3-{5-[(2-fluorophenyl)amino]-1H-indazol-1-yl}-N-(3,4,5-trimethoxyphenyl)benzamide | C29 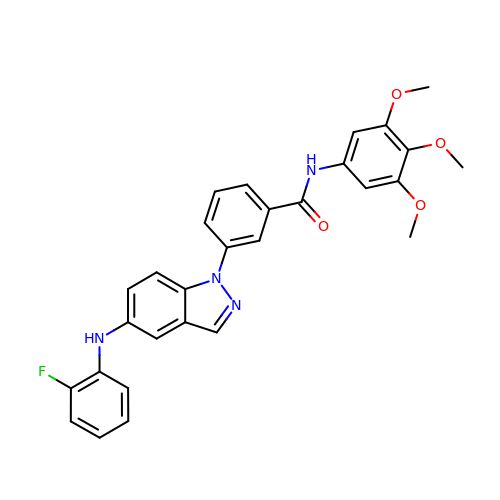H25 F N4 O4 | GYQLVKWGHKBDMP-UHFFFAOYSA-N AsfvLIG catalyzes the DNA ligation reaction during the base excision repair (BER) process of ASFV genome. AsfvLIG is composed of 419 amino acids and is one of the smallest DNA ligases identified to date. However, unlike the homologous proteins (such as HsLIG1 and SusLIG1), the fidelity of AsfvLIG is very low. By solving four AsfvLIG:DNA complex structures, including the non-catalytic open form and the catalytic closed forms, we showed that the NTD, AD, and OB domains of AsfvLIG undergo a large conformational change during the catalytic assembly.

One unsealed C:G pair, one unsealed C:T pair, and one sealed C:T pair were, respectively, captured at the catalytic sites of the three catalytic form structures, referred to as AsfvLIG:CG, AsfvLIG:CT1, and AsfvLIG:CT2 hereafter. Our structures represent several different states of the reaction: the AsfvLIG:CG complex structure captured the Watson–Crick C:G pair prior to ligation, whereas AsfvLIG:CT1 and AsfvLIG:CT2 captured the mismatched C:T pair prior to and after the ligation process, respectively. The structures belong to two different space groups: P212121 for AsfvLIG:CT2 and P21 for both AsfvLIG:CG and AsfvLIG:CT1. However, as indicated by the low root mean square deviation values (rmsd, about 0.75 Å based on the superposition of 404 pairs of Cα atoms) among them, the three complex structures are very similar to each other. Unlike the extended non-catalytic structure, AsfvLIG undergoes large domain rearrangement and adopts a closed conformation in the catalytic AsfvLIG:DNA complex. AsfvLIG is assembled like a ring-shaped clamp and encircles the DNA duplex in its central channel. Though not identical, the overall shapes and orientations of the C:T pair in AsfvLIG:CT1 and the C:G pair in AsfvLIG:CG are similar. Mismatched C:T pair and Watson–Crick C:G pair have similar conformations in the AsfvLIG:CT1 and AsfvLIG:CG structures.

> SMLNQFPGQYSNNIFCFPPIESETKSGKKASWIICVQVVQHNTIIPITDEMFSTDVKDAVAEIFTKFFVEEGAVRISKMTRVTEGKNLGKKNATTVVHQAFKDALSKYNRHARQKRGAHTNRGMIPPMLVKYFNIIPKTFFEEETDPIVQRKRNGVRAVACQQGDGCILLYSRTEKEFLGLDNIKKELKQLYLFIDVRVYLDGELYLHRKPLQWIAGQANAKTDSSELHFYVFDCFWSDQLQMPSNKRQQLLTNIFKQKEDLTFIHQVENFSVKNVDEALRLKAQFIKEGYEGAIVRNANGPYEPGYNNYHSAHLAKLKPLLDAEFILVDYTQGKKGKDLGAILWVCELPNKKRFVVTPKHLTYADRYALFQKLTPALFKKHLYGKELTVEYAELSPKTGIPLQARAVGFREPINVLEII>[6x]MSNATKFGKVAVLLGGKSAERAVSLDSGQAVLDALLRSGVQAEAFDPQDRSVTELVNYDRAFIVLHGRGGEDGQIQGVLEWLNIPYTGTGVQG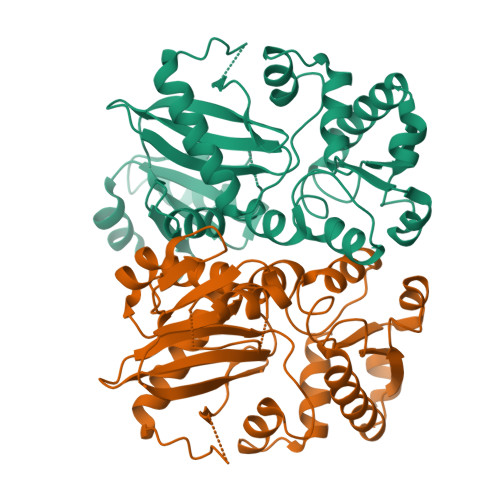SAIGMDKVKTKQIWQGSDLPTAPYRIITKETDLDSVIAELGLPVIIKPVHEGSSVGMSKVEKAEDFAAAIEKATQHDAVVMAEKWITGREFTISFLNGQPLPVIRLQPPADVAFYDYEAKYQRNDVEYGIPCGLSETEEKKLQALCLRAFQAVGAEGWGRIDAMQDEQGNFWLLEVNTVPGMTSHSLVPKAAKAVGYSFDELCVAILEQTLEGTA> MSLVNGRRRTAASVVALTAALTALAALC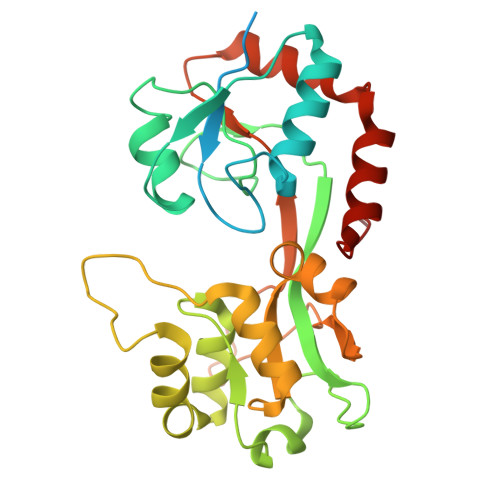APAQAQDTKATSKAAEAAKPDAGTLRVCAAEQPPLSMKDGSGLENRIATTVAEAMGRKAQFVWLGKPAIYLVRDGLEKKTCDVVIGLDADDPRVLTSKPYYRSGYVFLTRADKDLDIKSWSDPRLKEVSHMVVGFGTPGEAMLKDIGRYEEDMAYLYSLVNFRAPRNQYTQIDPARMVSEVATGKAEVGVAFGPDVARYVRDSSTKLRMTPVPDDTQASDGRKMPQSFDQAMGVRKDDTALKAEIDAALEKAKPKIEAILKEEGVPVLPVSN> METIDSKQNINRESLLEERRKKLAKWKQKKAQFDAQKEHQTSRNDIVTNSLEGKQTTEKFTERQERVKEELRKRKNEFRKSDEPVSVKPSKKKSKRSKVKKKISFDFSDDDDSEIGVSFRSKEHIQKAPEHDNEKDPLDEFMTSLKEEKMSNSKGMYDRGDILDVEDQLFELGGTDDEDVEDNTDNSNIAKIAKLKAKKRVKQIYYSPEELEPFQKNFYIESETVSSMSEMEVEELRLSLDNIKIKGTGCPKPVTKWSQLGLSTDTMVLITEKLHFGSLTPIQSQALPAIMSGRDVIGISKTGSGKTISYLLPLLRQVKAQRPLSKHETGPMGLILAPTRELALQIHEEVTKFTEADTSIRSVCCTGGSEMKKQI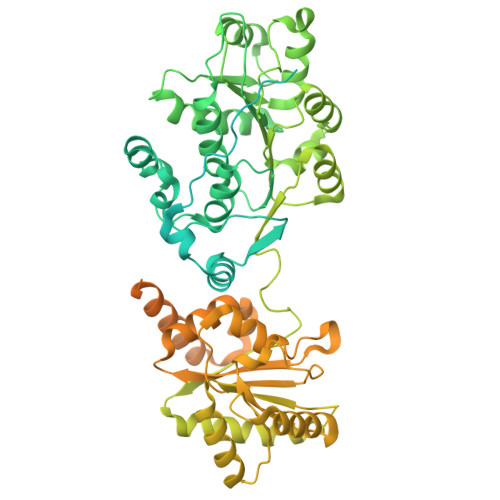TDLKRGTEIVVATPGRFIDILTLNDGKLLSTKRITFVVMDEADRLFDLGFEPQITQIMKTVRPDKQCVLFSATFPNKLRSFAVRVLHSPISITINSKGMVNENVKQKFRICHSEDEKFDNLVQLIHERSEFFDEVQSENDGQSSDVEEVDAKAIIFVSSQNICDFISKKLLNAGIVTCAIHAGKPYQERLMNLEKFKREKNSILLCTEVLSRGLNVPEVSLVIIYNAVKTFAQYVHTTGRTARGSRSGTAITLLLHDELSGAYILSKAMRDEEIKALDPLQAKELQEMSAKFESGMKKGKFRLSKGFGGKGLENIKSKREEAQNKDLELKKNDKRSDDLEKKISNPREGHDSVSESSALIPRLNYELFKESTDGSIIFYAKVYINDLPQIVRWEATKNTTLLFIKHETGCSITNKGKFYPEGKEPKNENDEPKLYLLIEGQDEKDIQLSIELLEQKVKEGVVKAASLSLKSTKY>MTRDQNGTWEMESNENFEGYMKALDIDFATRKIAVRLTQTKVIDQDGDNFKTKTTSTFRNYDVDFTVGVEFDEYTKSLDNRHVKALVTWEGDVLVCVQKGEKENRGWKQWIEGDKLYLELTCGDQVCRQVFKK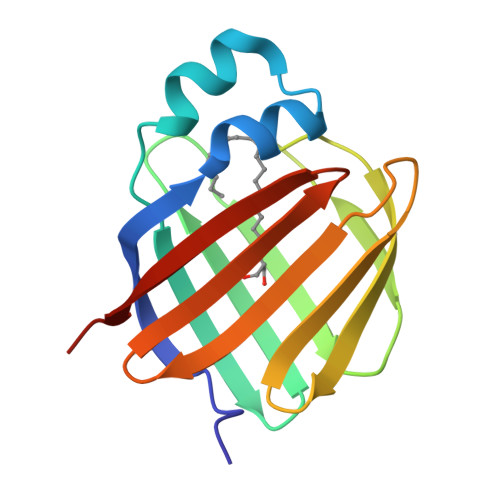KLVPR[2x]>MKGTIFAVALNHRSQLDAWQEAFQQSPYKAPPKTAVWFIKPRNTVIGCGEPIPFPQGEKVLSGATVALIVGKTATKVREEDAAEYIAGYALANDVSLPEESFYRPAIKAKCRDGFCPIGETVALSNVDNLTIYTEINGRPADHWNTADLQRNAAQLLSALSEFATLNPGDAILLGTPQARVEIQPGDRVRVLAEGFPPLENPVVDEREVTTRKSFPTLPHPHGTLFALGLNYADHASELEFKPPEEPLVFLKAPNTLTGDNQTSVRPNNIEYMHYEAELVVVIGKQARNVSEADAMDYVAGYTVCNDYAIRDYLENYYRPNLRVKSRDGL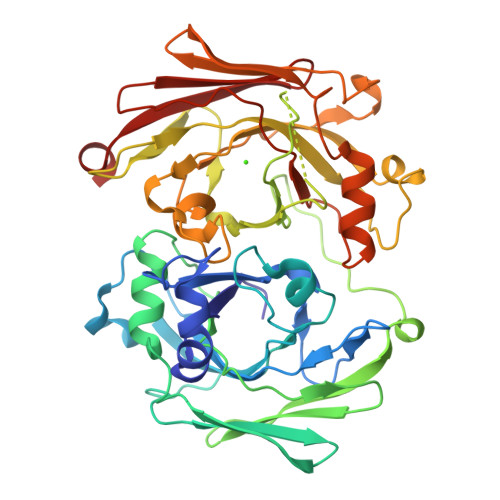TPMLSTIVPKEAIPDPHNLTLRTFVNGELRQQGTTADLIFSVPFLIAYLSEFMTLNPGDMIATGTPKGLSDVVPGDEVVVEVEGVGRLVNRIVSEETAK[4x]> GGGAGUACGGUGAGGGUCGGGU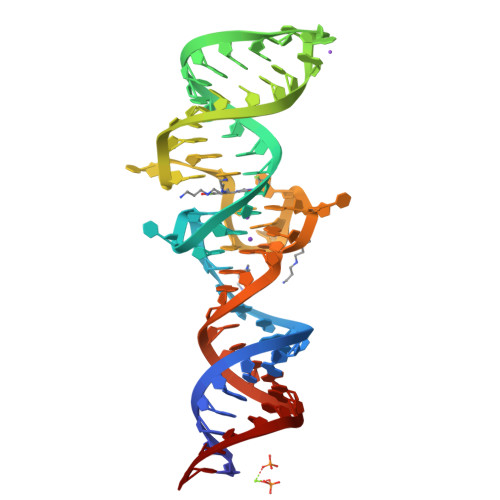CCAGUAGGUACGCCUACUGUUGAGUAGAGUGUGGGCUCCGUACUCCC4-(chloromethyl)benzoic acid | C8 H7 Cl O2 | 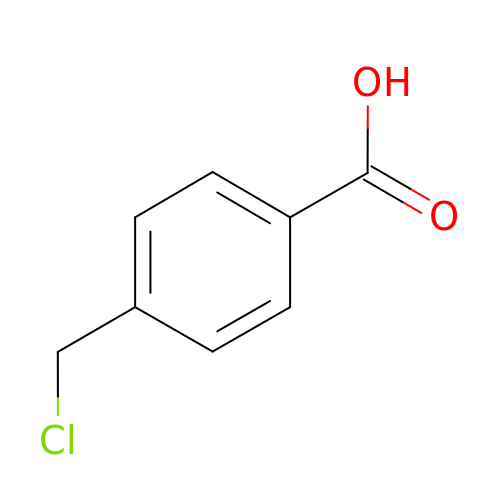OITNBJHJJGMFBN-UHFFFAOYSA-N>[2x]MGETLPNLRVEKLEEGV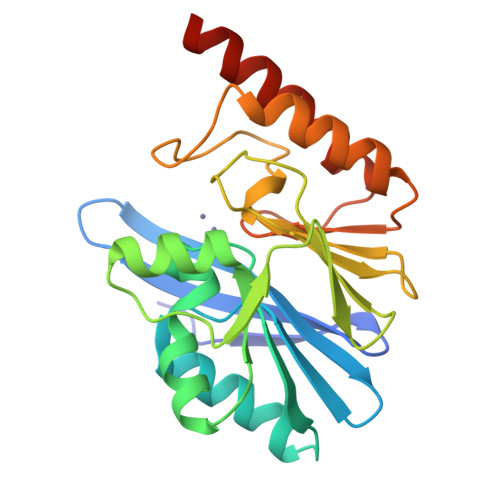YVHTSYEEVKGWGVVTKHGLVVLIGADAYLIDTPFTAKDTEKLVNWFVERGYKIKGTVSSHFHSDSTGGIEWLNSQSIPTYASELTNELLKKDGKVQAKNSFDGVSYWLAKDKIEVFYPGPGHTQDNVVVWLPEKEILFGGCFVKPHGLGNLGDANLEAWPESAKILMEKYGKAKLVVSGHSETGDATHLKRTWEQAVKGLKESKKTLQPSN> ARINGP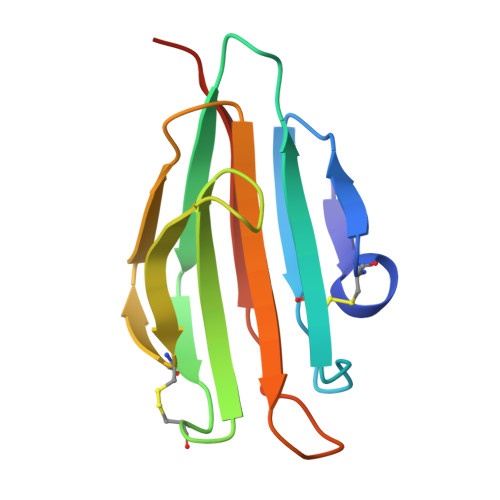DECGRVIKDTSGSISNTDRQKNLCTWTILMKPDQKVRMAIPYLNLACGKEYVEVFDGLLSGPSYGKLCAGAAIVFLSTANTMTIKYNRISGNSSSPFLIYFYGSSPGSEY>[2x]SNSKEITAQSQRHILNQSDHLRIDYELTRESMTKLRLVIFYSNISSDPITNFALLVASPKGTTLSLQPQSGN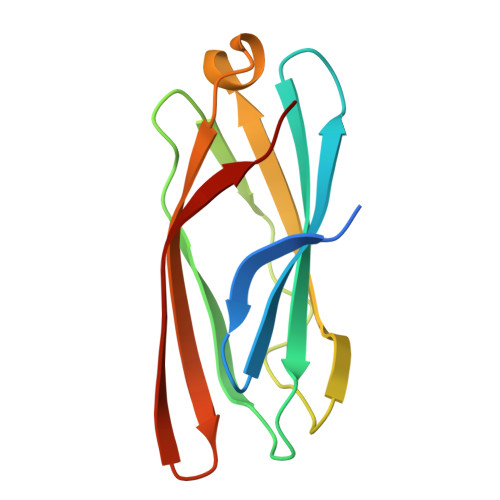MLQSNSRDGIKQIASVEGISVNLGKPIKLKWKANYCTKGDSKEESGTTSLPTI> MLNPTFSLYRKTLQSYPVPPKIRHYDRRWSGSRTNPYNRQYWRVIMNENYSRPSFWVSDFRHRYLMRTGTDYQ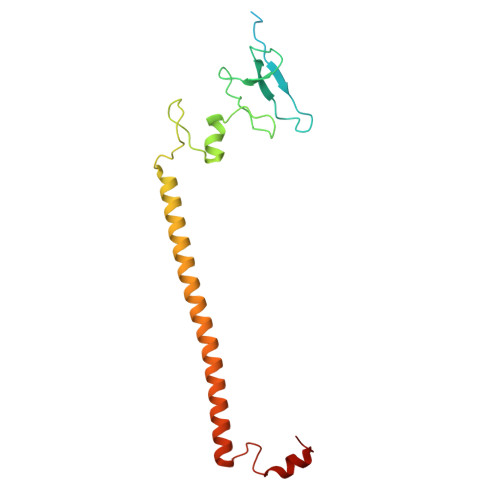GQVPSSPQPGLYQGFSDVHKLLANHPKPQRESRHLPVLPMTPRIVFEHANEKRIDTAKRMRRDRRRIEELKTLEFWGWYMKLQRVRGRWCREQGVSSRGVYGPAVDAAELWG>[2x]MNGAELIIQEINKEAERKIEYILNEAR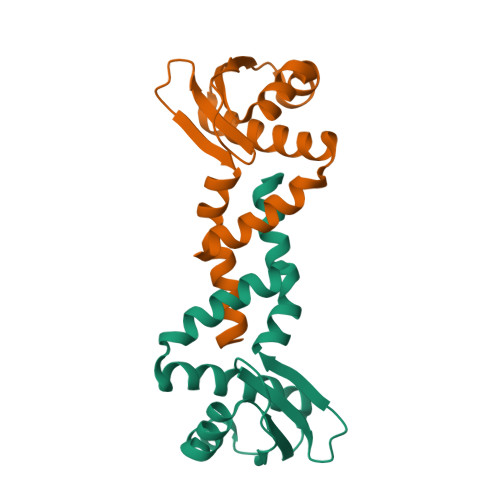QQAEKIKEEARRNAEAKAEWIIRRAKTQAELEKQRIIANARLEVRRKRLAIQEEIISSVLEEVKRRLETMSEDEYFESVKALLKEAIKELNEKKVRVMSNEKTLGLIASRIEEIKSELGDVSIELGETVDTMGGVIVETEDGRIRIDNTFEARMERFEGEIRSTIAKVLFG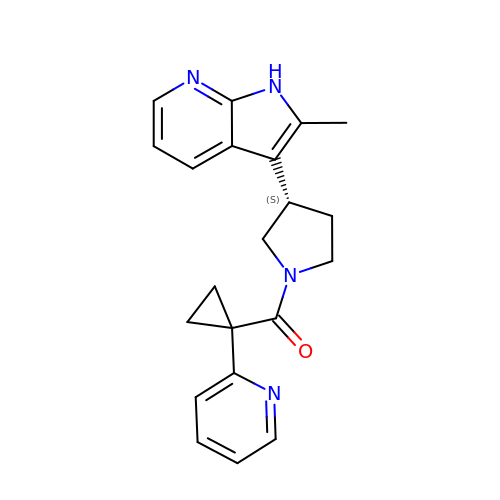2-methyl-3-{(3S)-1-[(1-pyridin-2-ylcyclopropyl)carbonyl]pyrrolidin-3-yl}-1H-pyrrolo[2,3-b]pyridine | C21 H22 N4 O | HUWRMRPEILCPLL-OAHLLOKOSA-N> AGVMTGAKFTQIQFGMTRQQVLDIAGAENCETGGSFGDSIHCRGHAAGDYYAYATFGFTSAAADAKVDSKSQEKL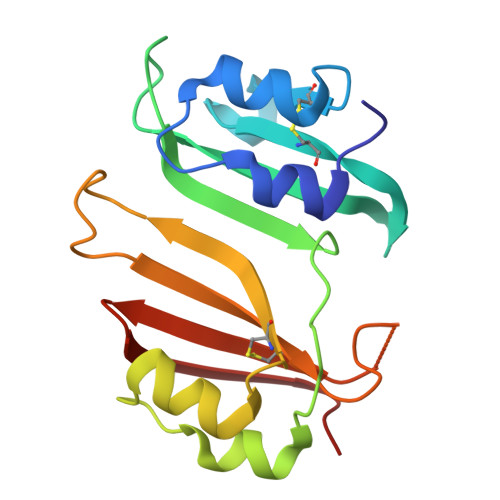LAPSAPTLTLAKFNQVTVGMTRAQVLATVGQGSCTTWSEYYPAYPSTAGVTLSLSCFDVDGYSSTGFYRGSAHLWFTDGVLQGKRQWDLV4-[(6-cyanonaphthalen-1-yl)oxy]-3-[2-(2,4-dioxo-3,4-dihydropyrimidin-1(2H)-yl)ethoxy]phenyl sulfurofluoridate | C23 H16 F 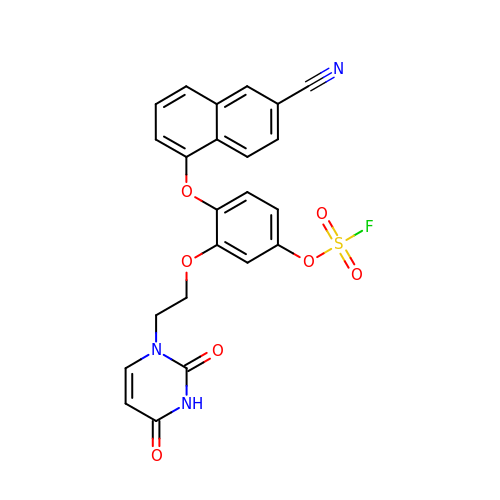N3 O7 S | XVIQCYUMLUTRMI-UHFFFAOYSA-N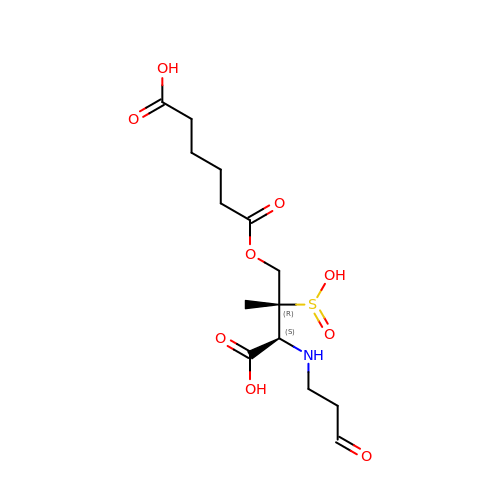6-({(2R,3S)-3-carboxy-2-methyl-3-[(3-oxopropyl)amino]-2-sulfinopropyl}oxy)-6-oxohexanoic acid | C14 H23 N O9 S | XJDMDWLRMVEPAR-JSGCOSHPSA-N>[6x]MIDVMQIQEILPHRYPFLLVDKITELKVKEVVLGYKNISISDHVFMGHFPGHPIYPGVLILEGMAQTGGVLAFESME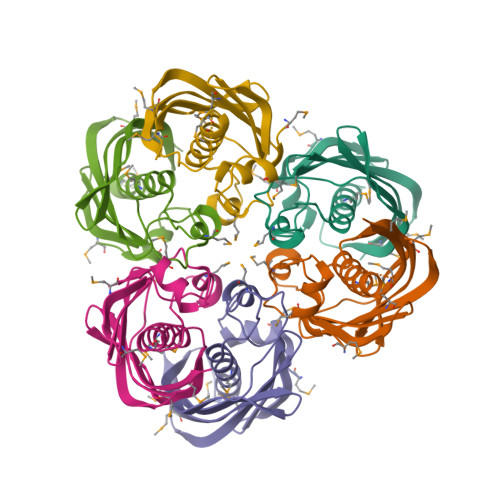DKVDPKSKVVYFTGIDGAKFRNPVRPGDRLDYEMSVVKNRGNMWIFKGQAFVDGNLVAEAELKAMIVDK> W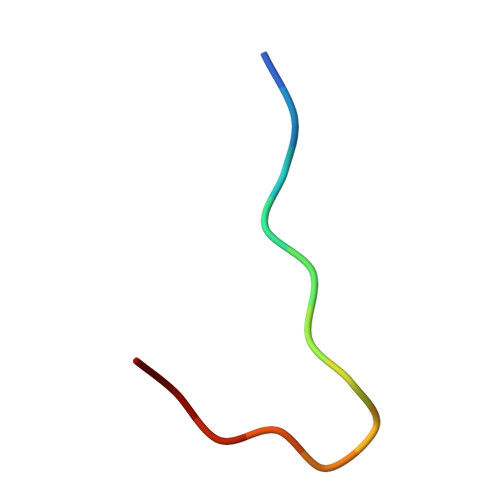HWLQLKPGQPMY>[2x]MHHHHHHARATGKTFRSGNSEAVRLPRDLA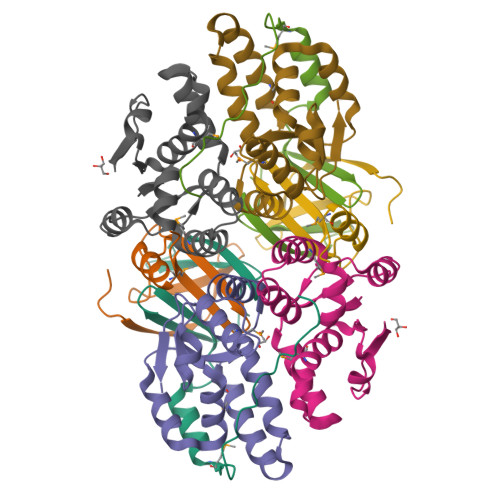FGADVELTLIRSGDVLTIYPSKGSIADLVATLNQMPRPDSVEIRDEDLFPERPGL;>MAYVLDTNVAIHLRDGDPEVTTRVTALNGAILLSIISRVELEGGVYREAAQAGLRRSRLDVMLKVLPVLDFDGAAADEYRRIVESAGYSRRKVVDRMIAAQALAHRATFVTFNADDFRDIPGLSLLAW[2x]>MENSEKTEVVLLACGSFNPITNMHLRLFELAKDYMNGTGRYTVVKGIISPVGDAYKKKGLIPAYHRVIMAELATKNSKWVEVDTWESLQKEWKETLKVLRHHQEKLEASDCDHQQNSPTLERPGRKRKWTETQDSSQKKSLEPKTKAVPKVKLLCGADLLESFAVPNLWKSEDITQIVANYGLICVTRAGNDAQKFIYESDVLWKHRSNIHVVNEWIANDISSTKIRRALRRGQSIRYLVPDLVQEYIEKHNLYSSESEDRNAGVILAPLQRNTAEAKT[6x];>MQANGAGGGGGGGGGGGGGGGGGGGQGQTPELACLSAQNGESSPSSSSSAGDLAHANGLLPSAPSAASNNSNSLNVNNGVPGGAAAASSATVAAASATTAASSSLATPELGSSLKKKKRLSQSDEDVIRLIGQHLNGLGLNQTVDLLMQESGCRLEHPSATKFRNHVMEGDWDKAENDLNELKPLVHSPHAIVRMKFLLLQQKYLEYLEDGKVLEALQVLRCELTPLKYNTERIHVLSGYLMCSHAEDLRAKAEWEGKGTASRSKLLDKLQTYLPPSVMLPPRRLQTLLRQAVELQRDRCLYHNTKLDNNLDSVSLLIDHVCSRRQFPCYTQQILTEHCNEVWFCKFSNDGTKLATGSKDTTVIIWQVDPDTHLLKLLKTLEGHAYGVSYIAWSPDDNYLVACGPDDCSELWLWNVQTGELRTKMSQSHEDSLTSVAWNPDGKRFVTGGQRGQFYQCDLDGNLLDSWEGVRVQCLWCLSDGKTVLASDTHQRIRGYNFEDLTDRNIVQEDHPIMSFTISKNGRLALLNVATQGVHLWDLQDRVLVRKYQGVTQGFYTIHSCFGGHNEDFIASGSEDHKVYIWHKRSELPIAELTGHTRTVNCVSWNPQIPSMMASASDDGTVRIWGPAPFIDHQNIEEECSSMDS[2x]

Here, we discover that human WDR26 binds the metabolic enzyme NMNAT1 and mediates its CTLH E3-dependent ubiquitylation independently of canonical GID/CTLH E3-family substrate receptors. Cryo-EM structures of NMNAT1- and YPEL5-bound WDR26-CTLH E3 assemblies reveal an internal basic degron motif of NMNAT1 essential for targeting by WDR26-CTLH E3, and degron mimicry by YPEL5’s N-terminus antagonizing substrate targeting. Cryo-EM structures reveal that WDR26 acts as a non-interchangeable substrate receptor for NMNAT1. Within the supramolecular WDR26-CTLH E3 assembly, the WD40-repeat β-propeller domains from two WDR26 dimers are exposed and provide multiple binding surfaces for NMNAT1.

All visualized NMNAT1-bound WDR26-CTLH E3 assemblies form giant hollow oval structures centrally encapsulating the hexameric NMNAT1 substrate, overall resembling the yeast Chelator-GIDSR4 E3 encapsulating its tetrameric Fbp1 substrate. However, unlike in the Chelator-GIDSR4 E3 where dual substrate receptor Gid4 subunits bind N-terminal degrons of tetrameric Fbp1, the data suggested that the centrally facing β-propeller domains of the WDR26 dimers mediate NMNAT1 recruitment, thereby positioning multiple solvent-exposed NMNAT1 lysines in proximity to CTLH E3 catalytic domains. A 3.8-Å-resolution map obtained by focused refinement enabled placing atomic coordinates for the β-propeller domains of the WDR26 dimer on one side of the complex interacting with a pair of globular NMNAT1 core domains from neighboring protomers in the NMNAT1 hexamer. The NMNAT1 core domain does not fully cover the β-propeller surface but rather docks on its largely hydrophobic edge. Here, the loops within and between four WDR26 blades establish interactions with three NMNAT1 helices, which are distal to the NMNAT1 active sites. Nicotinamide-mononucleotide (NMN) is bound to NMNAT1 in the focused-refined map. Notably, the prior structures of substrate, product, and a NAD+-mimetic drug-bound NMNAT1 are superimposable and can be docked onto the WDR26-bound complex, suggesting that recognition of NMNAT1 by WDR26-CTLH E3 would not be affected by occupancy of its active site. Substituting the WDR26-interacting NMNAT1 core residues with alanines (core>A) only subtly impaired NMNAT1 ubiquitylation and binding to WDR26-CTLH E3, suggesting that other interactions anchor the complex. Notably, a motif we term NMNAT1basic due to its consisting of three basic residues (K126, R127 and K128), anchors WDR26. Thus, the internal basic motif within NMNAT1’s disordered loop is critical for targeting NMNAT1 to the WDR26-CTLH E3.> GKDGSTAVPSLVALEKINVADIINGAQEKCVLPPMDGYPHCEGKIKWMKDMWRSDPCYADYGVDGSTCSFFIYLSEVENWCPHLPWRAKNPYEEADHNSLAEIRTDFNILYSMMKKHEEFRWMRLRIRRMADAWIQAIKSLAEKQNLEKRKRKKVLVHLGLLTKESGFKIAETAFSGGPLGELVQWSDLITSLYLLGHDIRISASLAELKEIMKKVVGNRSGCPTVGDRIVELIYIDIVGLAQFKKTLGPSWVHYQCMLRVLDSFGTEPEFNHANYAQSKGHKTPWGKWNLNPQQFYTMFPHTPDNSFLGFVVEQHLNSSDIHHINEIKRQNQSLVYGKVDSFWKNKKIYLDIIHTYMEVHATVYGSSTKNIPSYVKNHGILSGRDLQFLLRETKLFVGLGFPYEGPAPLEAIANGCAFLNPKFNPPKSSKNTDFFIGKPTLRELTSQHPYAEVFIGRPHVWTVDLNNQEEVEDAVKAILNQKIEPYMPYEFTCEGMLQRINAFIEKQDFCHGQVMWPPLSALQVKLAEPGQSCKQVCQESQLICEPSFFQHLNKDKDMLKYKVTCQSSELAKDILVPSFDPKNKHCVFQGDLLLFSCAGAHPRHQRVCPCRDFIKGQVALCKDCL

Human GnT-V is a type II membrane protein and comprises 741 amino acids in total. GnT-V acts only on the α1-6 mannose branch of N-glycans, and this process is highly regulated. Mechanistically, the β1-6 branch glycan modification by GnT-V allows target proteins to be decorated with a number of N-acetyllactosamine (LacNAc) residues, creating high-affinity ligands for galectins. In this study, we determined the crystal structures of the GnT-V catalytic domain in an apo form and in complex with our bisubstrate-type inhibitor as a substrate analog.

We tested a series of constructs truncating the N-terminal region and found T121-L741, named GnT-V luminal domain, is sufficient for catalytic reaction without impairing protein production in mammalian cells. We determined the crystal structure of GnT-V luminal domain (T121-L741) in apo form at 1.9 Å resolution by the native single-wavelength anomalous diffraction (SAD) method. Overall structure of GnT-V luminal domain has a cross-like shape and is composed of four subdomains: N-terminal domain (A128-Y207 in blue and G337-P339 in cyan in Fig. 2a), middle domains 1 (H212-K329 and I345-L424 in green, and E606-H627 in yellow) and 2 (G425-Y605 in orange), and C-terminal domain (G628-L741 in pink). As both of the two middle domains take Rossmann folds, GnT-V is classified into the GT-B fold. As the other human GnTs also require a divalent cation for catalysis, GnT-V is unique among human GnTs. The four subdomains of GnT-V luminal domain do not exist independently but instead are tightly connected by two short insertions (shown in cyan and yellow in Fig. 2a), as well as interregional disulfide bonds such as C172-C338 and C372-C626. And, the N-terminal domain is linked to middle domain 1 via three missing loop regions, signifying the highly mobile nature of this domain. GnT-V luminal domain contains eight disulfide bonds in total and five of them are located at the C-terminal domain. In the crystal structure, only one N-glycan was assigned at N433. E297 is located at the lid of the cleft formed by the two middle domains and is likely well positioned to act as a catalytic base.> NRSLNELSLSDILIAADVEGGLHAVDRRNGHIIWSIEPENFQPLIEIQEPSRLETYETLIIEPFGDGNIYYFNAHQGLQKLPLSIRQLVSTSPLHLKTNIVVNDSGKIVEDEKVYTGSMRTIMYTINMLNGEIISAFGPGSKNGYFGSQSVDCSPEEKIKLQECENMIVIGKTIFELGIHSYDGASYNVTYSTWQQNVLDVPLALQNTFSKDGMCIAPFRDKSLLASDLDFRIARWVSPTFPGIIVGLFDVFNDLRTNENILVPHPFNPGDHESISSN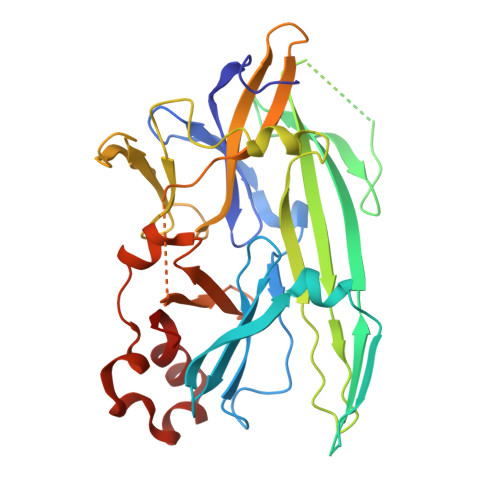KVYLDQTSNLSWFALSSQNFPSLVESAPISRYASSDRWRVSSIFEDETLFKNAIMGVHQIY[(1S)-1-(3,4-dichlorophenyl)-3-{hydroxy[2-(1H-1,2,4-triazol-1-ylmethyl)benzoyl]amino}propyl]phosphonic 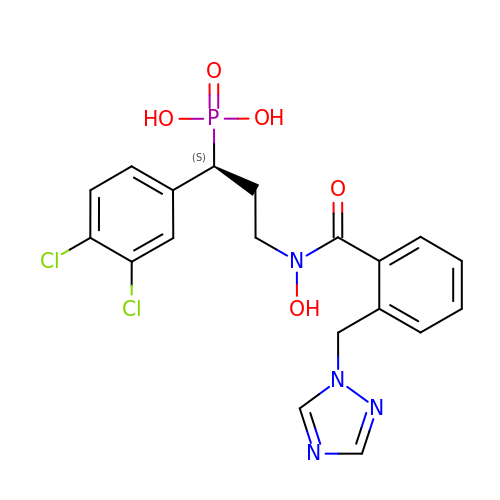acid | C19 H19 Cl2 N4 O5 P | CGKYBZFXVQNZBL-SFHVURJKSA-N> EVVKLLLEHGAD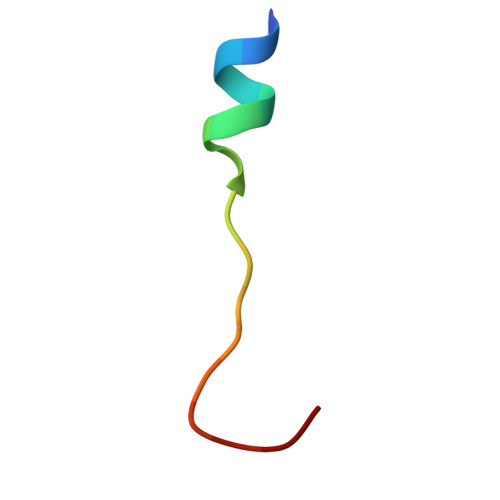VLAQD However, for these theories to be broadly applicable, they need to be demonstrated for large and multimeric enzymes that catalyze complicated reactions. The enzyme used in this study is a type II DNA topoisomerase (Top2) from African swine fever virus (Asfv), a dimeric multi-subdomain enzyme (271 kDa) that catalyzes multistep reactions to modulate DNA topology. AsfvTop2 has been found to be involved in the early stage of viral gene replication, and also detected at the intermediate and late stages of infection. The domain composition of AsfvTop2 resembles that of the canonical Type IIA DNA topoisomerases (Top2), including the well-studied eukaryotic counterparts, which form homodimers. The catalytic process not only involves well-coordinated changes in protein quaternary structures to allow timely opening and closing of the N-, DNA-, and C-gates, but also ATP binding and sequential hydrolysis that relate the dimerization and catalytic activity of the ATPase domain to the mechanistic steps of the cycle.

Furthermore, the ATPase domain of AsfvTop2 in the MgAMP-PNP-bound crystal structures coexist in reduced and oxidized forms involving a disulfide bond, which can regulate the AsfvTop2 function. Next we address a new regulatory mechanism unique to AsfvTop2. The crystal structure of AsfvTop2 ATPase domain obtained from a non-reducing condition was solved at 1.14 Å resolution (with density maps in Supplementary Fig. 12). Structural analysis indicates that the structures from reducing and non-reducing conditions are without and with a C72-C138 disulfide bond, respectively. Interestingly, the disulfide bond formation involves a large movement of C72 to reach C138, along with relocation of H73 to pair with D137. Additionally, this significant movement led to partial deformation of helix-α2. The formation of disulfide bond between C72-C138 and the involvement of H73 are supported by mass spectrometry and NMR, respectively. Kinetic assays further indicated that the ATP hydrolysis activity was significantly dampened upon oxidation. Thus, formation of the C72-C138 disulfide bond is most likely a naturally occurring way, in place of mutation, to enable the regulation of the ATPase activity and presumably the topoisomerase function. Importantly, this disulfide bond-mediated regulation of ATPase activity has not been shown in other Top2 enzymes. In line with the redox regulation of AsfvPolX and AsfvAP, formation of the disulfide bond by the cysteine pair (C72-C138) of AsfvTop2 can lower the activity of the topoisomerase, thus also save the ATP consumption and slow down DNA replication and cell growth, all of which may favor survival of the virus in under oxidative stress.

> MEAFEISDFKEHAKKKSMWAGALNKVTISGLMGVFTEDEDLMALPIHRDHCPALLKIFDELIVNATDHERACHSKTKKVTYIKISFDKGVFSCENDGPGIPIAKHEQASLIAKRDVYVPEVASCFFLAGTNINKAKDCIKGGTNGVGLKLAMVHSQWAILTTADGAQKYVQQINQRLDIIEPPTITPSREMFTRIELMPVYQELGYAEPLSETEQADLSAWIYLRACQCAAYVGKGTTIYYNDKPCRTGSVMALAKMYTLLSAPNSTIHTATIKADAKPYSLHPLQVAAVVSPKFKKFEHVSIINGVNCVKGEHVTFLKKTINEMVIKKFQQTIKDKNRKTTLRDSCSNIFVVIVGSIPGIEWTGQRKDELSIAENVFKTHYSIPSSFLTSMTRSIVDILLQSISKKD> KEQTSFNNPEPMTGFEHTVT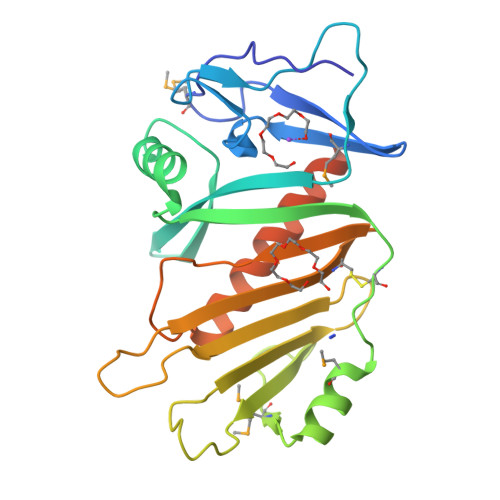FDFQGTKMVIPYGYLARYTQDNATKWLSDTPGQDAYSINLIEISVYYKKTDQGWVLEPYNQQNKAHFIQFLRDGLDSVDDIVIRKDACSLSTTMGERLLTYGVKKMPSAYPEYEAYEDKRHIPENPYFHEFYYIKKGENPAIITHRNNRINQTEEDSYSTSVGSCINGFTVQYYPFIREKQQLTQQELVGYHQQVEQLVQSFVNNSNKKENLYFQGLEHHHHHH(3S,6S)-3-(3,4-dihydroxybenzyl)-6-(4-hydroxybenzyl)piperazine-2,5-dione | C18 H18 N2 O5 | 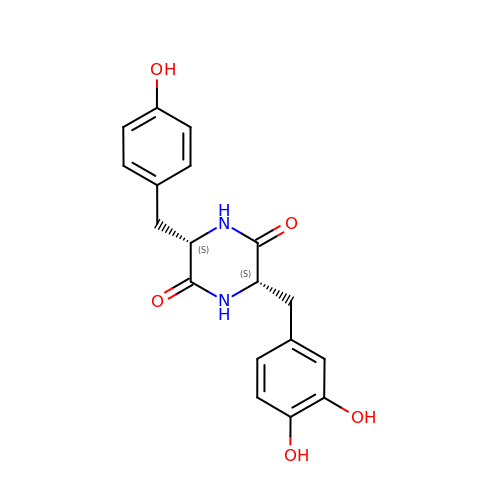OCFXXSJPAMPFJD-KBPBESRZSA-N3-[2-({4-[(2-amino-4-oxo-4,7-dihydro-3H-pyrrolo[2,3-d]pyrimidin-5-yl)methyl]benzene-1-carbonyl}amino)phenyl]propanoic acid | C23 H21 N5 O4 | 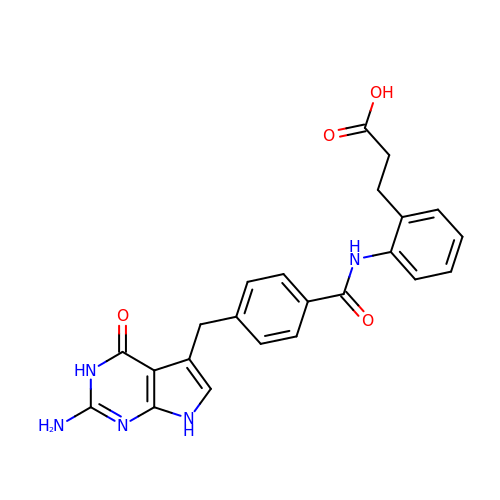PABYCMRDFQGQKT-UHFFFAOYSA-N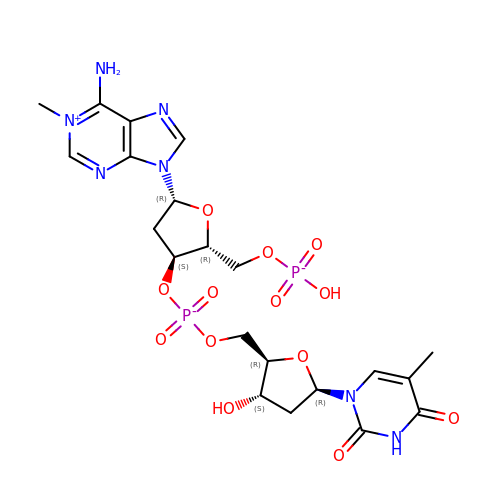[(3~{S},5~{R})-5-(6-azanyl-1-methyl-purin-9-yl)-2-(phosphonooxymethyl)oxolan-3-yl] [(2~{R},3~{S},5~{R})-5-[5-methyl-2,4-bis(oxidanylidene)pyrimidin-1-yl]-3-oxidanyl-oxolan-2-yl]methyl hydrogen phosphate | C21 H28 N7 O13 P2 | AESRSXSUEFZXFW-KPRKPIBOSA-O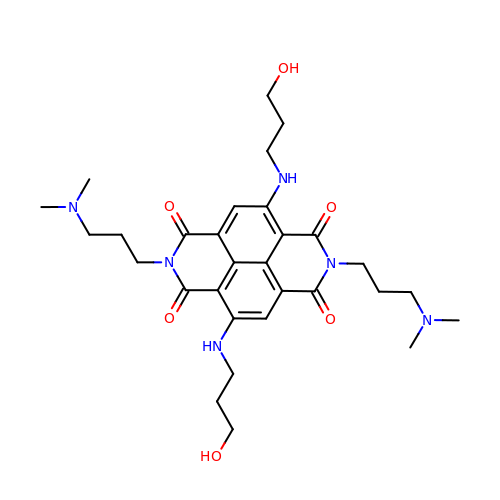2,7-bis[3-(dimethylamino)propyl]-4,9-bis[(3-hydroxypropyl)amino]benzo[lmn][3,8]phenanthroline-1,3,6,8(2H,7H)-tetrone | C30 H42 N6 O6 | XRDZCSQPAUGHQH-UHFFFAOYSA-N>[9x]MLGSLVLRRKALAPRLLLRLLRSPTLRGHGGASGRNVTTGSLGEPQWLRVATGGRPGTSPALFSGRGAATGGRQGGRFDTKCLAAATWGRLPGPEETLPGQDSWNGVPSRAGLGMCALAAALVVHCYSKSPSNKDAALLEAARANNMQEVSRLLSEGADVNAKHRLGWTAL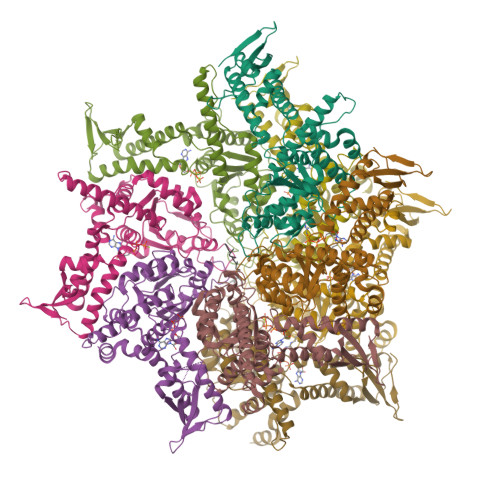MVAAINRNNSVVQVLLAAGADPNLGDDFSSVYKTAKEQGIHSLEVLITREDDFNNRLNNRASFKGCTALHYAVLADDYRTVKELLDGGANPLQRNEMGHTPLDYAREGEVMKLLRTSEAKYQEKQRKREAEERRRFPLEQRLKEHIIGQESAIATVGAAIRRKENGWYDEEHPLVFLFLGSSGIGKTELAKQTAKYMHKDAKKGFIRLDMSEFQERHEVAKFIGSPPGYVGHEEGGQLTKKLKQCPNAVVLFDQVDKAHPDVLTIMLQLFDEGRLTDGKGKTIDCKDAIFIMTSNVASDEIAQHALQLRQEALEMSRNRIAENLGDVQISDKITISKNFKENVIRPILKAHFRRDEFLGRINEIVYFLPFCHSELIQLVNKELNFWAKRAKQRHNITLLWDREVADVLVDGYNVHYGARSIKHEVERRVVNQLAAAYEQDLLPGGCTLRITVEDSDKQLLKSPELPSPQAEKRLPKLRLEIIDKDSKTRRLDIRAPLHPEKVCNTI>[2x]MGGVSDERLDLVNERDEVVGQILRTDPALRWERVRVVNAFLRNSQGQLWIPRRSPSKSLFPNALDVSVGGAVQSGETYEEAFRREAREELNVEIDALSWRPLASFSPFQTTLSSF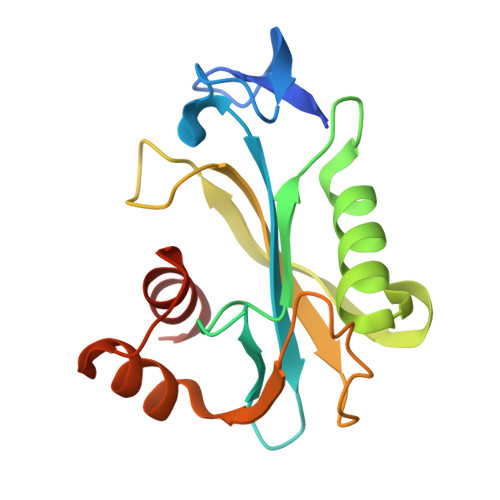MCVYELRSDATPIFNPNDISGGEWLTPEHLLARIAAGEAAKGDLAELVRRCYREEE> MAAHQMDSITYSNNVTQQYIQPQSLQDISAVEDEIQNKIEAARQESKQLHAQINKAKHKIQDASLFQMANKVTSLTKNKINLKPNIVLKGHNNKISDFRWSRDSKRILSASQDGFMLIWDSASGLKQNAIPLDSQWVLSCAISPSSTLVASAGLNNNCTIYRVSKENRVAQNVASIFKGHTCYISDIEFTDNAHILTASGDMTCALWDIPKAKRVREYSDHLGDVLALAIPEEPNSENSSNTFASCGSDGYTYIWDSRSPSAVQSFYVNDSDINALRFFKDGMSIVAGSDNGAINMYDLRSDCSIATFSLFRGYEERTPTPTYMAANMEYNTAQSPQTLKSTSSSYLD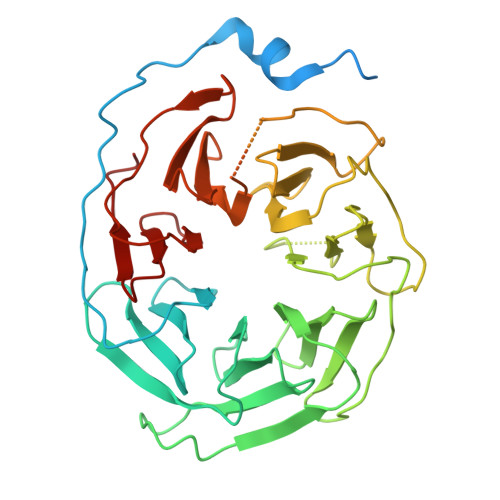NQGVVSLDFSASGRLMYSCYTDIGCVVWDVLKGEIVGKLEGHGGRVTGVRSSPDGLAVCTGSWDSTMKIWSPGYQ>[2x]SANENNL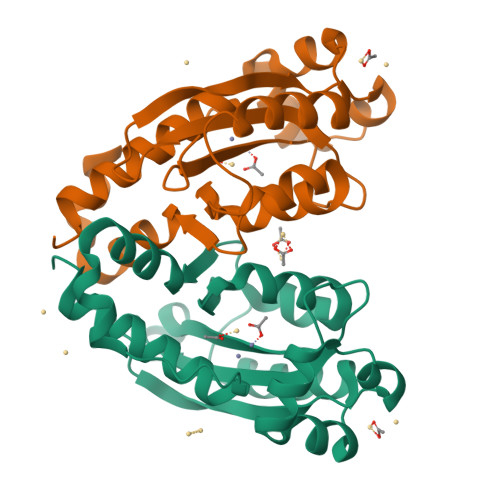IWIDLEMTGLDPERDRIIEIATLVTDANLNILAEGPTIAVHQSDEQLALMDDWNVRTHTASGLVERVKASTMGDREAELATLEFLKQWVPAGKSPICGNSIGQDRRFLFKYMPELEAYFHYRYLDVSTLKELARRWKPEILDGFTKQGTHQAMDDIRESVAELAYYREHFIKL> AR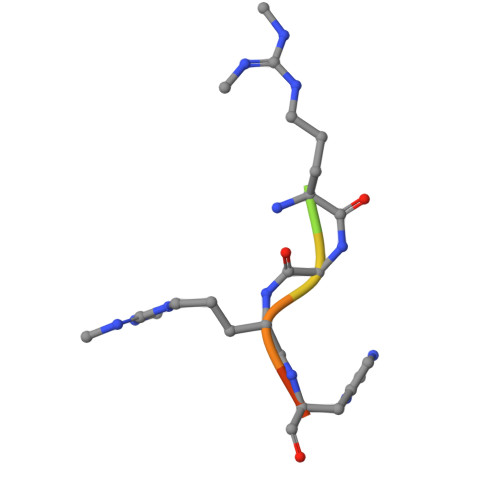GRGRHPG Human SIDT1 and SIDT2 are closely related members of the SID-1 transmembrane family, and have been implicated in various biological processes such as glucose and lipid metabolism, innate immunity, and tumorigenesis. Here, we present the cryo-electron microscopy (cryo-EM) structures of human SIDT1 and SIDT2. Both structures reveal an overall architecture of a dimeric arrangement composed of an extracellular domain (ECD) rich in β-strands and a transmembrane domain (TMD) with 11 passes, highlighting the remarkable structural congruence. Importantly, the ECDs of SIDT1 and SIDT2 bind synthetic plant-derived miRNA only under acidic conditions.

SIDT2 mainly localizes to the lysosomal membrane. It can facilitate the uptake of naked single-stranded (ss) oligonucleotides into cells, and mediate RNA/DNA uptake by lysosomes during RNautophagy/DNautophagy. We first solved cryo-EM structures of SIDT1 and SIDT2 at overall resolutions of 3.33 Å and 3.17 Å, respectively. The electron density maps exhibited well-defined main-chain connectivity and side-chain densities in the ECDs, while the TMDs have relatively lower quality and resolution. Both SIDT1 and SIDT2 form homodimeric structures involving their ECD and TMD, exhibiting a high degree of symmetry with a two-fold rotational axis perpendicular to the membrane surface. SIDT2 also contains ten predicted N-glycosylation sites, with all six glycosylation sites on its ECD well resolved in the EM map, along with the corresponding disulfide bonds. Furthermore, SIDT2 features an additional β-strand (residues 27–33) involved in interactions at the dimer interface, while the corresponding region in SIDT1 remains unstructured, indicating a high level of flexibility and fewer interactions at the dimer interface of SIDT1 compared to SIDT2. In the SIDT2 ECD model, the dimerization interaction involves a buried surface area of ~1700 Å2 from each protomer, in contrast to ~1300 Å2 in the SIDT1 model, indicating differences in the proximity of the formed homodimers between SIDT1 and SIDT2, probably due to sequence variations. In contrast, SIDT2 relies more on interactions between TM2 and TM6 for dimerization. Cryo-EM structures of SIDT1 and SIDT2 show highly conserved features despite only 57% sequence identity.

>[2x]MKANLLVLLCALAAADAHLGVLGPKNVSQKDAEFERTYVDEVNSELVNIYTFNHTVTRNRTEGVRVSVNVLNKQKGAPLLFVVRQKEAVVSFQVPLILRGMFQRKYLYQKVERTLCQPPTKNESEIQFFYVDVSTLSPVNTTYQLRVSRMDDFVLRTGEQFSFNTTAAQPQYFKYEFPEGVDSVIVKVTSNKAFPCSVISIQDVLCPVYDLDNNVAFIGMYQTMTKKAAITVQRKDFPSNSFYVVVVVKTEDQACGGSLPFYPFAEDEPVDQGHRQKTLSVLVSQAVTSEAYVSGMLFCLGIFLSFYLLTVLLACWENWRQKKKTLLVAIDRACPESGHPRVLADSFPGSSPYEGYNYGSFENVSGSTDGLVDSAGTGDLSYGYQGRSFEPVGTRPRVDSMSSVEEDDYDTLTDIDSDKNVIRTKQYLYVADLARKDKRVLRKKYQIYFWNIATIAVFYALPVVQLVITYQTVVNVTGNQDICYYNFLCAHPLGNLSAFNNILSNLGYILLGLLFLLIILQREINHNRALLRNDLCALECGIPKHFGLFYAMGTALMMEGLLSACYHVCPNYTNFQFDTSFMYMIAGLCMLKLYQKRHPDINASAYSAYACLAIVIFFSVLGVVFGKGNTAFWIVFSIIHIIATLLLSTQLYYMGRWKLDSGIFRRILHVLYTDCIRQCSGPLYVDRMVLLVMGNVINWSLAAYGLIMRPNDFASYLLAIGICNLLLYFAFYIIMKLRSGERIKLIPLLCIVCTSVVWGFALFFFFQGLSTWQKTPAESREHNRDCILLDFFDDHDIWHFLSSIAMFGSFLVLLTLDDDLDTVQRDKIYVFDYKDHDGDYKDHDIDYKDDDDK> SRLNRESVIDAALELLNETGIDGLTTRKLAQK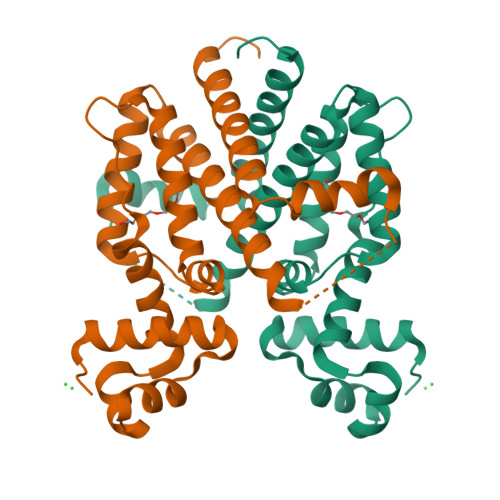LGIEQPTLYWHVKNKRALLDALAVEILARHHDYSLPAAGESWQSFLRNAAMSFRRALLRYRDGAKVHLGTRPDEKQYDTVETQLRFMTENGFSLRDGLYAISAVSHFTLGAVLEQQEHTAALTDRPAAPDENLPPLLREALQIMDSDDGEQAFLHGLESLIRGFEVQLTALLQIV URIDINE-5'-DIPHOSPHATE-XYLOPYRANOSE 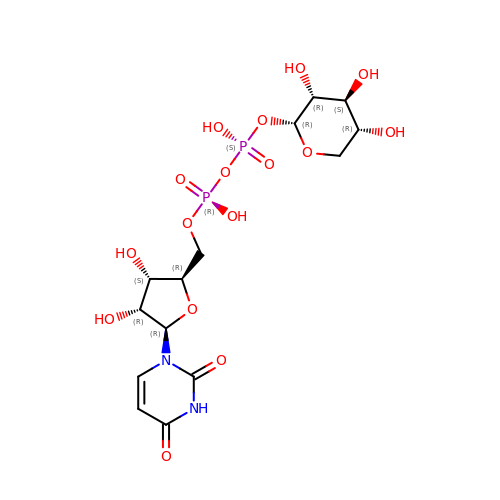| C14 H22 N2 O16 P2 | DQQDLYVHOTZLOR-OCIMBMBZSA-N> VMLTRQQKELIVKEMSEIFKKTSLILFADFLGFTVADLTELRSRLREKYGDGARFRVVKNTLLNLALKNAEYEGYEEFLKGPTAVLYVTEGDPVEAVKIIYNFYKDKKADLSRLKGGFLEGKKFTAEEVENIAKLPSKEELYAMLVGRVKAPITGL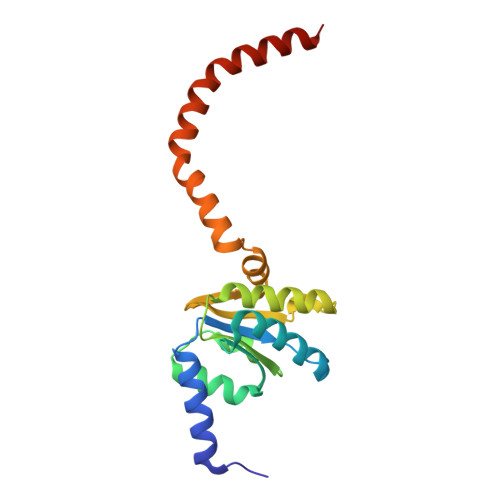VFALSGILRNLVYVLNAIKEKKSE> MQEGVKVVVDSRELRSEVVKRLKLLGVKLEVKTLDVGDYIISEDVAIERKSANDLIQSIIDGGLFDQVKRLKEAYSRPIMIVEGSLYGIRNVHPN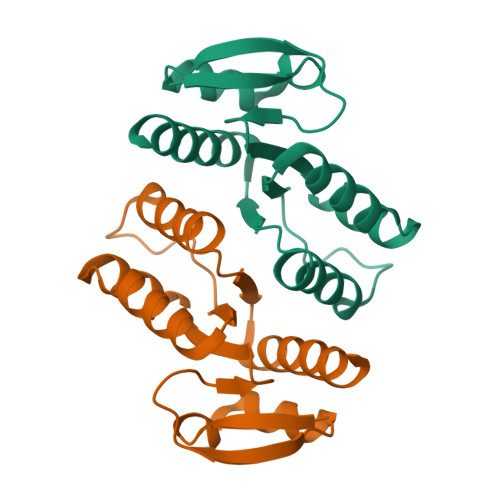AIRGAIAAVTVDFGVPIIFSSTPEETAQYIFLIAKREQEEREKPVRIR>[3x]GSGNIKTLGDAYEFAVDVRDFSPEDIIVTTSNNHI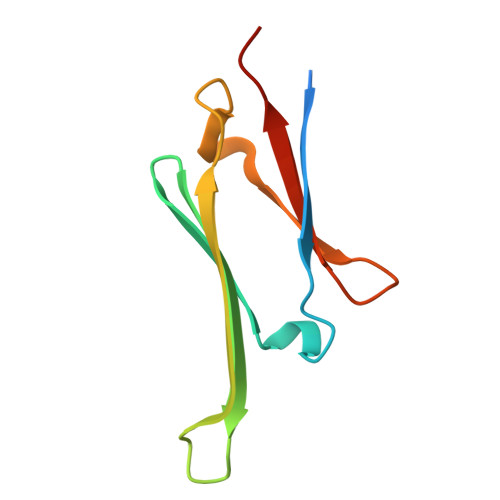EVRAEKLAADGTVMNTFAHKSQLPEDVDPTSVTSALREDGSLTIRARRHPHT>[2x]MLEGLSWVDYGERAELDDSDGHGNHRESSPFLSPLEASRGIDYYDRNLALFEEELDIRPKVSSLLGKLVSYTNLTQGAKEHEEAESGEGTRRRAAEAPSMG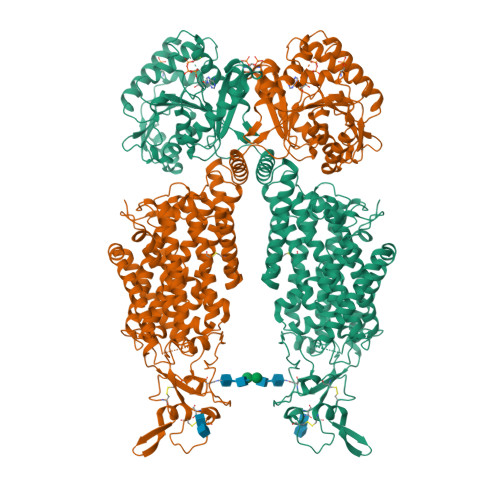TLMGVYLPCLQNIFGVILFLRLTWMVGTAGVLQALLIVLICCCCTLLTAISMSAIATNGVVPAGGSYFMISRSLGPEFGGAVGLCFYLGTTFAAAMYILGAIEILLTYIAPPAAIFYPSGAHDTSNATLNNMRVYGTIFLTFMTLVVFVGVKYVNKFASLFLACVIISILSIYAGGIKSIFDPPVFPVCMLGNRTLSRDQFDICAKTAVVDNETVATQLWSFFCHSPNLTTDSCDPYFMLNNVTEIPGIPGAAAGVLQENLWSAYLEKGDIVEKHGLPSADAPSLKESLPLYVVADIATSFTVLVGIFFPSVTGIMAGSNRSGDLRDAQKSIPVGTILAIITTSLVYFSSVVLFGACIEGVVLRDKYGDGVSRNLVVGTLAWPSPWVIVIGSFFSTCGAGLQSLTGAPRLLQAIAKDNIIPFLRVFGHGKVNGEPTWALLLTALIAELGILIASLDMVAPILSMFFLMCYLFVNLACAVQTLLRTPNWRPRFKYYHWALSFLGMSLCLALMFVSSWYYALVAMLIAGMIYKYIEYQGAEKEWGDGIRGLSLSAARYALLRLEEGPPHTKNWRPQLLVLLKLDEDLHVKYPRLLTFASQLKAGKGLTIVGSVIQGSFLESYGEAQAAEQTIKNMMEIEKVKGFCQVVVASKVREGLAHLIQSCGLGGMRHNSVVLGWPYGWRQSEDPRAWKTFIDTVRCTTAAHLALLVPKNIAFYPSNHERYLEGHIDVWWIVHDGGMLMLLPFLLRQHKVWRKCRMRIFTVAQMDDNSIQMKKDLAVFLYHLRLEAEVEVVEMHNSDISAYTYERTLMMEQRSQMLRQMRLTKTEREREAQLVKDRHSALRLESLYSDEEDESAVGADKIQMTWTRDKYMTETWDPSHAPDNFRELVHIKPDQSNVRRMHTAVKLNEVIVTRSHDARLVLLNMPGPPRNSEGDENYMEFLEVLTEGLERVLLVRGGGREVITIYSAENLYFQ> MASGQYNCPGQYTFSMPSDSHVSSCSEDWV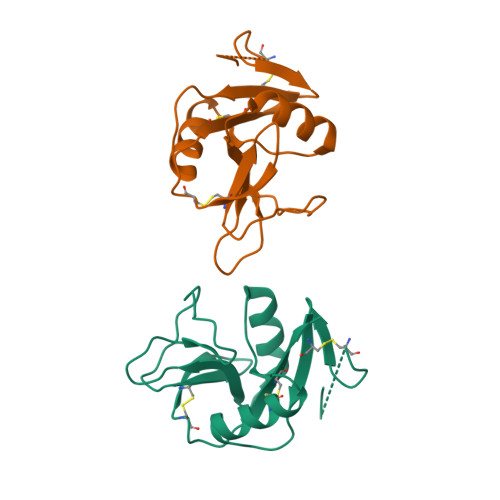GYQRKCYFISTVKRSWTSAQNACSEHGATLAVIDSEKDMNFLKRYAGREEHWVGLKKEPGHPWKWSNGKEFNNWFNVTGSDKCVFLKNTEVSSMECEKNLYWICNKPYK Proper operation of the pivotal CME cargo adaptor AP2 requires membrane-localized Fer/Cip4 homology domain-only proteins (FCHO). The AP2 complex, composed of α, β2, μ2, and σ2 subunits, is pivotal to mammalian CCV formation, and its deletion is embryonically lethal in mice. FCHO1 and FCHO2 are similar in overall domain arrangement —folded N-terminal acidic phospholipid-binding homodimerization F-BAR domains and C-terminal folded μ-homology domains (μHD) separated by a ~300-residue, low-complexity intrinsically disordered protein linker, which has been suggested to participate in AP2 activation, although how it does so is undetermined. We dissect the network of interactions between the FCHO interdomain linker and AP2, which concentrates, orients, tethers, and partially destabilizes closed AP2 at the plasma membrane.

To confirm the identity of the extra, Cμ2-proximal electron density as the N terminus of FCHO2 linker, chimeras of Cμ2 alone with N1+N2 attached to the C terminus via 30-residue unstructured synthetic glycine-, serine-, and alanine-rich flexible linkers were then created, crystallized, and their structures solved at resolutions varying from 2.0 to 2.6 Å by MR using an unliganded version of Cμ2 as a search model. The Y pocket is variously filled by parts of the tags of an adjacent Cμ2 molecule. Muniscin family conserved side chains make key interactions with Cμ2 residues 167 to 170, which form the BR3 PtdIns(4,5)P2-binding site. The N1 interaction occurs mainly via complementary charged interactions between Asp318, Glu320, and Glu321 and the Cμ2 BR3 PtdIns(4,5)P2-binding site containing Lys167, Tyr168, and Arg169. Isothermal titration calorimetry (ITC) measurements showed the binding of FCHO2-N1+N2 to have a KD of ~25 μM. Mutation of key binding residues in Cμ2 (E320A+E321A+K326A) reduced binding fivefold, and mutating Tyr323 to serine rendered it unmeasurably weak. The FCHO linker does not directly interact with the Y or Ø cargo motif binding pockets in any structure but does pass close by before its main chain changes direction at FCHO2 Pro327. The weak density that follows on from N1 adopts a range of conformations forming crystal packing contacts, which we believe to be nonphysiological (mutations FCHO2 Y340S and E336A+F339S have little effect on N1-N2 binding). Whereas N1+N2 binds Cμ2 with a KD of around 25 μM, N1 alone (i.e., deletion of N2) reduces binding by ~5-fold, demonstrating that N2 plays a role in binding AP2. In support of this, mutating four of BR4’s basic residues to alanines (BR4-) caused substantial reduction in binding of GST·FCHO2 linker to Cμ2: The lower level of binding reduction of Serinc3 loop results from binding Cμ2 only at BR4 and not to BR3 (43), whereas in FCHO2, N1 can still bind to BR3 even when the BR4:N2 interaction is disrupted.

>PGIHMQIGWRREGIKYRRNELFLDVLESVNLLMSPQGQVLSAHVSGRVVMKSYLSGMPECKFGMNDKIVIEKQGKGTADETSKSGKQSIAIDDCTFHQCVRLSKFDSERSISFIPPDGEFELMRYRTTKDIILPFRVIPLVREVGRTKLEVKVVIKSNFKPSLLAQKIEVRIPTPLNTSGVQVICMKGKAKYKASENAIVWKIKRMAGMKESQISAEIELLPTNDKKKWARPPISMNFEVPFAPSGLKVRYLKVFEPKLNYSDHDVIKWVRYIGRSGIYETRCGASGSAGSAGPSGAGSAGSAGPSAGSAGSAGSGSAGSAPGPDVDEEGYSIKPETNQNDTKENHFYSSSDSDSEDEE[2x]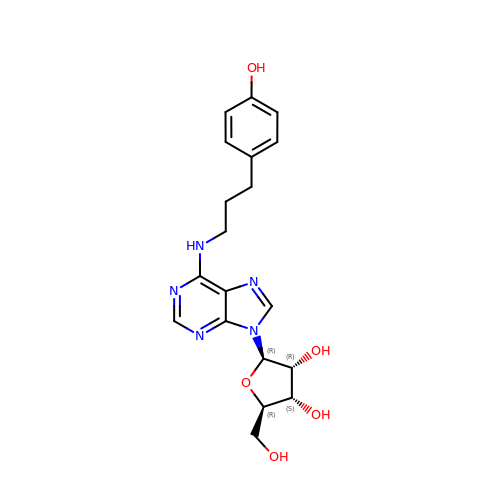N-[3-(4-hydroxyphenyl)propyl]adenosine | C19 H23 N5 O5 | UNEQRQPOYXLYJS-NVQRDWNXSA-N> NDPIANAVESAVSALADTTISRVTAANTTASTHSLGTGRVPALQAAETGASSNASDENLVETRCVMNRNGVNEASVEHFYSRAGLVGVVEVKDSGTSLDGYTVWPIDVMGFVQQRRKLELSTYMRFDAEFTFVSNLSNSTTPGMLLQYMYVPPGAPKPDGRKSYQWQTATNPSVFAKLSDPPPQVSVPFMSPATAYQWFYDGYPTFGEHKQATNLQYGQCPNNMMGHFAIRTVSESTTGKNVHVRVYMRIKHVRAWVPRPLRSQAYMVKNYPTYSQTITNTATDRASITTTDYEGGVPASPQRTS;> SPSVEACGYSDRVAQLTVGNSTITTQEAANIVLSYGEWPEYCPSTDATAVDKPTRPDVSVNRFYTLSTKSWKTESTGWYWKFPDVLNDTGVFGQNAQFHYLYRSGFCMHVQCNASKFHQGALLVAAIPEFVIAASSPATKPNGRGLYPDFAHTNPGKDGQEFRDPYVLDAGIPLSQALVFPHQWINLRTNNCATIIMPYVNALPFDSALNHSNFGLVVIPISPLKYCNGATTEVPVTLTIAPLNSEFSGLRQAIKQ;> GFPTELKPGTNQFLTTDDGTSPPILPGFEPTPLIHIPGEFTSLLDLCQIETILEVNNTTGTIGVSRLLIPVRAQNNVDQLCASFQVDPGRNGPWQSTMVGQICRYYTQWSGSLKVTFMFTGSFMATGKMLIAYTPPGSAQPATREAAMLGTHIVWDFGLQSSVTLVIPWISNTHFRAVKIGGVYDYYATGIVTIWYQTNFVVPPDTPTEANIIALGAAQKNFTLKLCKDTDEIQQTAAYQ

Although highly effective vaccines exist for EV71, no vaccine is available for the global public health threats imposed by CVA6, which underscores the critical need for developing an effective vaccine. Here, we demonstrate the isolation of two stable CVA6 particles with excellent natural antigenicity: one empty (CVA6 procapsid) and the other infectious (CVA6 A-particle). The capsid structures of CVA6 procapsid and A-particle at near atomic (~3 Å) resolution both closely resemble those of the uncoating intermediates of other enteroviruses. The cryoEM structures of the CVA6 procapsid, A-particle, and A-particle-1D5 immune-complex we report here reveal atomic resolution details about molecular determinants in CVA6 related to virus neutralization, cell binding, and RNA release.

The bottom band had a λ260/λ280 absorbance ratio of 1.65 with particles sedimenting at 128S and composed of capsid proteins VP1, VP2, and VP3 but no VP4 (lane 3), and contained packaged genome as verified by negative staining. Hence, the bottom band unexpectedly contained particles more like uncoating intermediates (or A-particles) as opposed to mature virions of other picornaviruses. In addition, the high infectivity of the CVA6 A-particle was measured to be 3.6 × 107 TCID50/mg, which demonstrates that A-particles can infect cells efficiently. The above results indicate that the isolated CVA6 A-particle is biochemically similar to the uncoating intermediates of other picornaviruses, but functions as a mature virus that has a stable structure and is highly infectious. The CVA6 A-particle contains characteristic structural features that are typically attributed solely to picornavirus A-particles. These include large, open channels at the icosahedral 2-fold (2f-channel) and quasi 3-fold axes (q3f-channel), and a collapsed hydrophobic pocket beneath VP1 ‘canyon’. The 2f-channel in CVA6 has dimensions of 36 Å × 8 Å, which are both similar to that in the CVA16 A-particle and the EV71 A-particle, whereas the channel is closed in the EV71 virion. In contrast to other known enteroviruses, CVA6 A-particles display unique interactions between its capsid and the packaged genome. The cryoEM density map and atomic model of the A-particle together reveal that the N-termini of VP2 and VP3 interact with the genomic RNA near the icosahedral 2- and 5-fold axes, respectively. The N-termini of five VP3 subunits extend beneath the VP1 ‘cooling tower’ to form a well-defined annulus with the key residue P3 making close interactions with the genomic RNA. Here, the CVA6 A-particle examined in this study, unlike the classical, mature picornavirion and instead more like a stable uncoating intermediate, may require only minimal conformational change in its capsid to enable release of the genomic RNA.> PETRPNHTIYINNLNEKIKKDELKKSLHAIFSRFGQILDILVSRSLKMRGQAFVIFKEVSSATNALRSMQGFPFYDKPMRIQYAKTDSDIIAKMA

The catalytic activity of the HDV ribozyme is essential for viral replication and viral particle assembly inside the host cells. In addition, residue C75 (C76 in the antigenomic ribozyme) is essential for the cleavage reaction, and mutating C75 to any other base, especially uracil or guanine, inhibits the reaction. In this study, we have used these new techniques to correct and improve the cleaved and the cis-acting C75U-inhibited structures of the HDV ribozyme, which were originally solved over a decade ago.

The 1CX0 crystal structure of the HDV ribozyme self-cleaved product was one of the earliest ribozyme structures ever solved, at 2.3Å resolution, with R = 24.6% and Rfree = 27.9% as calculated by PHENIX. Notably, it exploited the ability of U1A-RBD protein to form crystal contacts, thereby facilitating crystal growth, by removing part of the P4 stem-loop of the genomic HDV ribozyme and replacing it with a U1A hairpin. By using a combination of PHENIX refinement, ERRASER corrections and hand rebuilding in Coot and in KiNG, we made multiple changes to the model that improved its agreement with the experimental data and its MolProbity statistics. The pucker corrections were particularly impressive; hand refits and the use of RNABC were initially successful in correcting only one of these ribose puckers, PDB residue 152, refitting the C3′-endo pucker as C2′-endo, while the other seven ribose puckers were each corrected to C2′-endo pucker only by using ERRASER. A close look at the electron density near U23 led us to model a second alternate conformation for this residue (see Results) similar to that seen in the inhibited structures. This suggests that release of the metal ion from the active site indeed makes U23 more flexible, but the residue can still sample a conformation similar to structures when cleavage is inhibited. Occupancy refinement assigns alternate A and alternate B 0.64 and 0.36 occupancy, respectively. The rebuild for each of those structures (in independent ERRASER runs) resulted in a reverse G25:U20 wobble base pair: for 1CX0, small movements of U20 enabled the base-pair hydrogen bonds, whereas in 1VC7, G25 was flipped from anti to syn conformation (along with geometry and ribose pucker corrections). The clashscore is reduced to 0.75, placing the new structure in the 100th percentile for its resolution range. The final R = 19.85% and Rfree = 24.08%, improved by 4.75 and 3.82%, respectively.(R)-4-((2-azaspiro[3.3]heptan-2-yl)methyl)-N-((1-(6-(benzylamino)pyrimidin-4-yl)-3-hydroxypiperidin-3-yl)methyl)benzamide 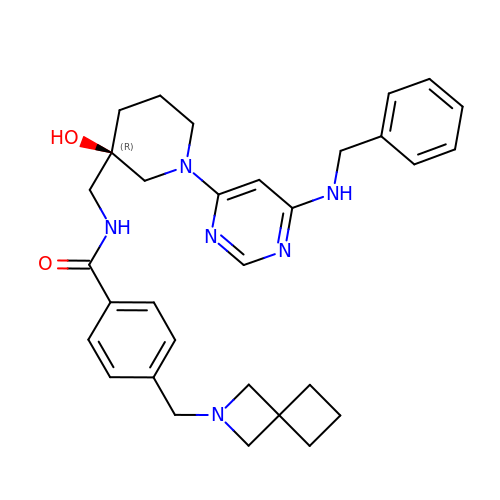| C31 H38 N6 O2 | YYXDDEFPSYEFQV-WJOKGBTCSA-N>[4x]VKLAGNSSLCPVSGWAPLSKDNSVRIGSKGDVFVIREPFISCSPLECRQFFLTQGALLNDKHSNGTIKDRSPYRTLMSVPIGSVPSPYNARFESIAWSASACHDGINWLTIGITGPDSGAVAILKYNGIITDTIKSWRNNILRTQESECACVNGSCFTIMTDGPSDGQASYKIFRIEKGKIIKSVEMKAPNYHYEECSCYPDSSEITCVCRDNWHGSNRPWVSFNQNLEYQMGYICSGVFGDNPRPNDKTGSCGPVSSNGANGVKGFSFKYGNGVWIGRTKSISSRKGFEMIWDPNGWTGTDNKFSIKQDIVGINEWSGYSGSFVMHPELTGLDCIVPCFWVELIRGRPEENTIWTSGSSISFCGVNSDTVGWSWPDGAELPFTIDK

NA is an enzyme that binds and cleaves sialosides from glycans on the host cell surface to facilitate the release of nascent viral particles from infected cells, and is also proposed to assist other stages in the virus replication cycle. NA is a homotetrameric, type II integral membrane protein with a short cytoplasmic N-terminal domain. Crystal structures of NA catalytic domains, either proteolytically released from virions or produced recombinantly, have consistently shown that four identical subunits interact non-covalently to form a globular “head” with four-fold symmetry. We use homology-directed protein design to uncover the structural principles underlying these distinct tetrameric conformations and stabilize multiple recombinant NAs in the “closed” state, yielding two near-atomic resolution structures of NA by cryo-EM.

To assess the portability of the closed state-stabilizing mutations, mutations from N1-CA09-sNAp-155 were introduced into the NA of N1 MI15, from the same post-2009 human lineage as CA09. We found that the sNAp-155 mutations clearly assisted stabilization of the closed state but were insufficient for complete closure, as N1-MI15-sNAp-155 adopted a mixture of the open and closed states. Given our hypothesis that E165S favors closure by making space D more ordered, we focused on redesigning the aqueous cavity surrounding D103, which is directly adjacent to residue 165 and another potential source of structural instability, in order to stabilize N1 MI15. Due to the higher yield of N1-MI15-sNAp-174 compared to the other designs and the simplicity of the single additional stabilizing mutation (T131Q), this design was selected for further analyses. Mirroring the results obtained with other sNAps, the stability of N1-MI15-sNAp-174 was relatively insensitive to Ca2+ and the Tm of the sNAp was 14.7 °C higher than N1-MI15-WT in the presence of EDTA. The Tagg was also higher in the presence of either Ca2+ or EDTA, and N1-MI15-sNAp-174 maintained the closed tetrameric state over a period of 15 days. We determined the structure of the N1-MI15-sNAp-174 tetramer at 3.2 Å resolution using cryo-EM. The structure, which strongly resembled the overall structure of N1-CA09-sNAp-155 (backbone RMSD of 0.77 and 0.80 Å over one and all four subunits of the tetramer, respectively), confirmed that N1-MI15-sNAp-174 adopts the closed tetrameric state in solution. The backbone rearrangement in space A observed in the N1-CA09-sNAp-155 structure was also found in N1-MI15-sNAp-174, along with a similar lack of density for the C-terminal regions, the 150-loop, and the 430-loop. The new T131Q mutation helps fill the space D cavity as intended while forming a hydrogen bond to the side chain of S442.>[3x]MDFSRNLYDIGEQLDSEDLASLKFLSLDYIPQRKQEPIKDALMLFQRLQEKRMLEESNLSFLKELLFRINRLDLLITYLNTRKEEMERELQTPGRAQISAYRVMLYQISEEVSRSELRSFKGGLQEEISKCKLDDDMNLLDIFIEMEKRVILGEGKLDILKRVCAQINKSLLKIINDYEEFSKERSSSLEGSPDEFSNGEELCGVMTISDSPREQDSESQTLDKVYQMKSKPRGYCLIINNHNFAKAREKVPKLHSIRDRNGTHLDAGALTTTFEELHFEIKPHDDCTVEQIYEILKIYQLMDHSNMDCFICCILSHGDKGIIYGTDGQEAPIYELTSQFTGLKCPSLAGKPKVFFIQAAQGDNYQKGIPVETASEEQPYLEMALSSPQTRYIPDEADFLLGMATVNNCVSYRNPAEGTWYIQSLCQSLRERCPRGDDILTILTEVNYEVSNKDDKKNMGKQMPQPTFTLRKKLVFPSD;>MSAEVIHQVEEALDTDE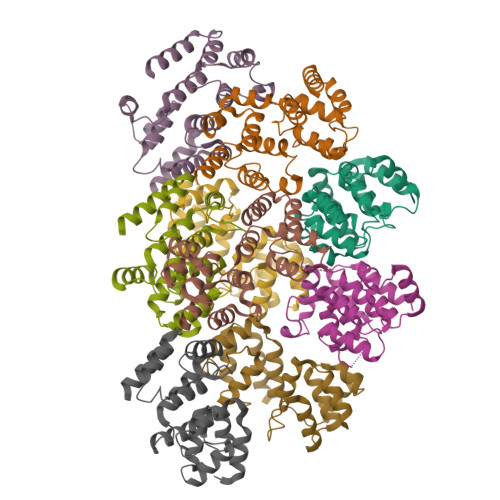KEMLLFLCRDVAIDVVPPNVRDLLDILRERGKLSVGDLAELLYRVRRFDLLKRILKMDRKAVETHLLRNPHLVSDYRVLMAEIGEDLDKSDVSSLIFLMKDYMGRGKISKEKSFLDLVVELEKLNLVAPDQLDLLEKCLKNIHRIDLKTKIQKYKQSVQGAGTS[6x]> ASHMFRKLAAESFGTFWLVFGGSGSAVLAAGFPELGIGFAGVALAFGLTVLTMAFAVGHISGGHFNPAVTIGLWAGGRFPAKEVVGYVIAQVVGGIVAAALLYLIASGKTGFDAAASGFASNGYGEHSPGGYSMLSALVVELVLSAGFLLVIHGATDKFAPAGFAPIAIGLACTLIHLISIPVTNTSVNPARSTAVAIFQGGWALEQL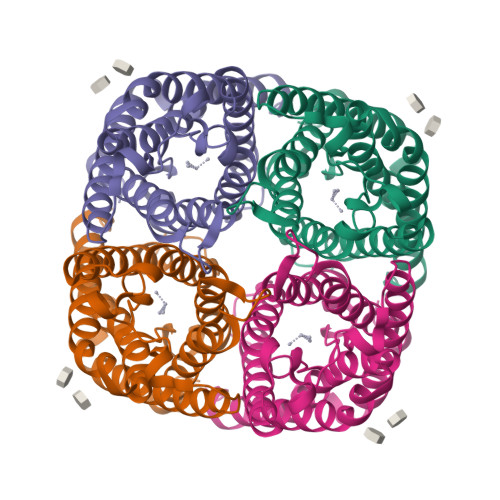WFFWVVPIVGGIIGGLIYRTLLEKRD>MLNQELELSLNMAFARAREHRHEFMTVEHLLLALLSNPSAREALEACSVDLVALRQELEAFIEQTTPVLPASEEERDTQPTLSFQRVLQRAVFHVQSSGRNEVTGANVLVAIFSEQESQAAYLLRKHEVSRLDVVNFISHGTRKDEPTQSSDPGSQPNSEEQAGGEERMENFTTNLNQLARVGGIDPLIGREKELERAIQVLCRRRKNNPLLVGESGVGKTAIAEGLAWRIVQGDVPEVMADCTIYSLDIGSLLAGTKYRGDFEKRFKALLKQLEQDTNSILFIDEIHTIIGAGAASGGQVDAANLIKPLLSSGKIRVIGSTTYQEFSNIFEKDRALARRFQKIDITEPSIEETVQIINGLKPKYEAHHDVRYTAKAVRAAVELAVKYINDRHLPDKAIDVIDEAGARARLMPVSKRKKTVNVADIESVVARIARIPEKSVSQSDRDTLKNLGDRLKMLVFGQDKAIEALTEAIKMARAGLGHEHKPVGSFLFAGPTGVGKTEVTVQLSKALGIELLRFDMSEYMERHTVSRLIGAPPGYVGFDQGGLLTDAVIKHPHAVLLLDEIEKAHPDVFNILLQVMDNGTLTDNNGRKADFRNVVLVMTTNAGVRETERKSIGLIHQDNSTDAMEEIKKIFTPEFRNRLDNIIWFDHLSTDVIHQVVDKFIVELQVQLDQKGVSLEVSQEARNWLAEKGYDRAMGARPMARVIQDNLKKPLANELLFGSLVDGGQVTVALDKEKNELTYGFQSAQKHKAEAAH[6x];>MSYSGERDNFAPHMALVPMVIEQTSRGERSFDIYSRLLKERVIFLTGQVEDHMANLIVAQMLFLEAENPEKDIYLYINSPGGVITAGMSIYDTMQFIKPDVSTICMGQAASMGAFLLTAGAKGKRFCLPNSRVMIHQPLGGYQGQATDIEIHAREILKVKGRMNELMALHTGQSLEQIERDT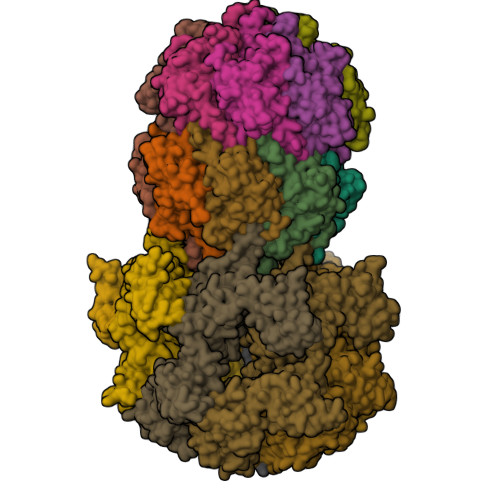ERDRFLSAPEAVEYGLVDSILTHRN[14x]> GSHMVMNTHPYQSEAVSDVWSLSKTSMTFQPKKASLQPLTISLDELFSSRGEFISVGGNGRMSHKEAILLGLRYKKLYNQ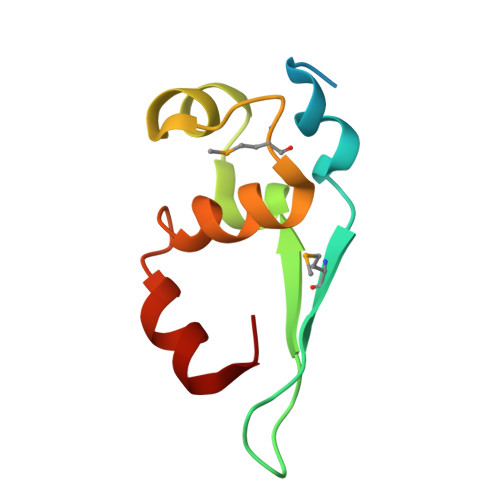ARVKYSL> MKFYIDDLPVLFPYPKIYPEQYNYMCDIKKTLDVGGNSILEMPSGTGKTVSLLSLTIAYQMHYPEHRKIIYCSRTMSEIEKALVELENLMDYRTKELGYQEDFRGLGLTSRKNLCLHPEVSKERKGTVVDEKCRRMTNGQAKRKLEEDPEANVELCEYHENLYNIEVEDYLPKGVFSFEKLLKYCEEKTLCPYFIVRRMISLCNIIIYSYHYLLDPKIAERVSNEVSKDSIVIFDEAHNIDNVCIESLSLDLTTDALRRATRGANALDERISEVRKVDSQKLQDEYEKLVQGLHSADILTDQEEPFVETPVLPQDLLTEAIPGNIRRAEHFVSFLKRLIEYLKTRMKVLHVISETPKSFLQHLKQLTFIERKPLRFCSERLSLLVRTLEVTEVEDFTALKDIATFATLISTYEEGFLLIIEPYEIENAAVPNPIMRFTCLDASIAIKPVFERFSSVIITSGTISPLDMYPRMLNFKTVLQKSYAMTLAKKSFLPMIITKGSDQVAISSRFEIRNDPSIVRNYGSMLVEFAKITPDGMVVFFPSYLYMESIVSMWQTMGILDEVWKHKLILVETPDAQETSLALETYRKACSNGRGAILLSVARGKVSEGIDFDHQYGRTVLMIGIPFQYTESRILKARLEFMRENYRIRENDFLSFDAMRHAAQCLGRVLRGKDDYGVMVLADRRFSRKRSQLPKWIAQGLSDADLNLSTDMAISNTKQFLRTMAQPTDPKDQEGVSVWSYEDLIKHQNSRKDQGGFIENENKEGEQDEDEDEDIEMQ;> MSHSGAAIFEKVSGIIAINEDVSPAELTWRSTDGDKVHTVVLSTIDKLQATPASSEKMMLRLIGKVDESKKRKDNEGNEVVPKPQRHMFSFNNRTVMDNIKMTLQQIISRYKDADIYEEKRRREESAQHTETPMSSSSVTAGTPTPHLDTPQLNNGAPLINTAKLDDSLSKEKLLTNLKLQQSLLKGNKVLMKVFQETVINAGLPPSEFWSTRIPLLRAFALSTSQKVGPYNVLSTIKPVASSENKVNVNLSREKILNIFENYPIVKKAYTDNVPKNFKEPEFWARFFSSKLFRKLRGEKIMQNDRGDVIIDRYLTLDQEFDRKDDDMLLHPVKKIIDLDGNIQDDPVVRGNRPDFTMQPGVDINGNSDGTVDILKGMNRLSEKMIMALKNEYSRTNLQNKSNITNDEEDEDNDERNELKIDDLNESYKTNYAIIHLKRNAHEKTTDNDAKSSADSIKNADLKVSNQQMLQQLSLVMDNLINKLDLNQVVPNNEVSNKINKRVITAIKINAKQAKHNNVNSALGSFVDNTSQANELEVKSTLPIDLLESCRMLHTTCCEFLKHFYIHFQSGEQKQASTVKKLYNHLKDCIEKLNELFQDV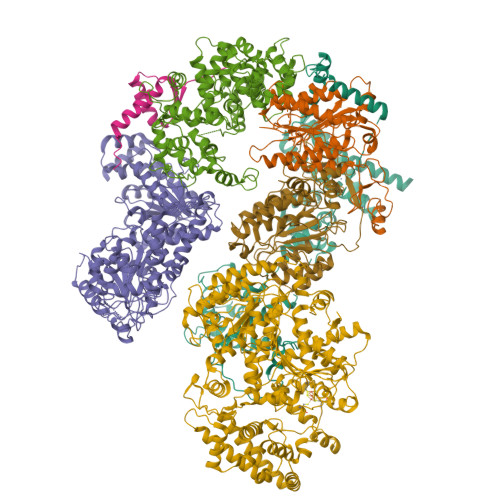LNGDGESMSNTCTAYLKPVLNSITLATHKYDEYFNEYNNNSN;> MSDYSLKHSVTQYLEEIPQQVQNRLYTSPATCLAIYRILPPLAKFFIMAMVFNENEVPLLDLDKWVNSNGKLQFQNAIKSMKSLHLLIPNKSSGTLMINLNPTFKISLRNALTGGEVQNSFGVVVEENVVSLDLLDEYSANKWETILHFMVGTPLAKIPSEKVLNLLKHSKLMEEVNSTGEFKITNEGFQFLLQEINSQLWTLLLQYLKMIETSKMDLVDVLHFIFMLGALEVGKAYKIDALSETQRIMLQDMRDYGLVFQKHSNDSIFYPTKLALMLTSDTKTIRSASNAMDSVLRQNREEPSVNEDGANGKSTTDITTSDDLNKAGLKNQDIPDGSLIVETNFKIYSYSNSPLQIAVLSLFVHLKARFVNMVLGQITRESIRRALTNGITADQIIAYLETHAHPQMRRLAEEKLEKKLELDPNCKEPLQVLPPTVVDQIRLWQLELDRVITYEGSLYSDFETSQEYNLLSKYAQDIGVLLWKDDKKKKFFISKEGNSQVLDFAKRKLKKKQ;> MDAISDPTFKHARSRKQVTEESPSLLTVIIEIAPKLWTTFDEEGNEKGSIIKVLEALIVFLNAHLAFNSANKVAVIAAYSQGIKYLYPESTSALKASESENKTRSDLKIINSDMYRRFRNVDETLVEEIYKLFELEKKQIEQNSQRSTLAGAMSAGLTYVNRISKESVTTSLKSRLLVLTCGSGSSKDEIFQYIPIMNCIFSATKMKCPIDVVKIGGSKESTFLQQTTDATNGVYLHVESTEGLIQYLATAMFIDPSLRPIIVKPNHGSVDFRTSCYLTGRVVAVGFICSVCLCVLSIIPPGNKCPACDSQFDEHVIAKLKRKPVVPRLKAKKKVTKP;> MARARKGALVQCDPSIKALILQIDAKMSDIVLEELDDTHLLVNPSKVEFVKHELNRLLSKNIYNPMDEEENQ;> MAPVVISESEEDEDRVAITRRTKRQVHFDGEGDDRVDQQQQQHSSSHRDRDKHVQRKKKKRLSNRNLQGSNGGYAWEDEIKRSWDLVKVDDEGDMASLVASIVEARKKRTAKKNITPYQRGIIRSLILTLDCSEAMLEKDLRPNRHAMIIQYAIDFVHEFFDQNPISQMGIIIMRNGLAQLVSQVSGNPQDHIDALKSIRKQEPKGNPSLQNALEMARGLLLPVPAHCTREVLIVFGSLSTTDPGDIHQTIDSLVSEKIRVKVLGLSAQVAICKELCKATNYGDESFYKILLDETHLKELFNEAVTPLPVNKINKGFTLVKMGFPTRIFEDTPTFCSCHSKLVYGGYFCPNCHSKVCSLPTVCPCCDLMLILSTHLARSYHHLMPLKTFAEVPTTEKFRSEDCFSCQSRFPILKNHKNGKLLTSSRYRCEDCKQEFCVDCDVFIHEILHNCPGCESKPVIT;> MTDVEGYQPKSKGKIFPDMGESFFSSDEDSPATDAEIDENYDDNRETSEGRGERDTGAMVTGLKKPRKKTKSSRHTAADSSMNQMDAKDKALLQDTNSDIPADFVPDSVSGMFRSHDFSYLRLRPDHASRPLWISPSDGRIILESFSPLAEQAQDFLVTIAEPISRPSHIHEYKITAYSLYAAVSVGLETDDIISVLDRLSKVPVAESIINFIKGATISYGKVKLVIKHNRYFVETTQADILQMLLNDSVIGPLRIDSDHQVQPPEDVLQQQLQQTAGKPATNVNPNDVEAVFSAVIGGDNEREEEDDDIDAVHSFEIANESVEVVKKRCQEIDYPVLEEYDFRNDHRNPDLDIDLKPSTQIRPYQEKSLSKMFGNGRARSGIIVLPCGAGKTLVGITAACTIKKSVIVLCTSSVSVMQWRQQFLQWCTLQPENCAVFTSDNKEMFQTESGLVVSTYSMVANTRNRSHDSQKVMDFLTGREWGFIILDEVHVVPAAMFRRVVSTIAAHAKLGLTATLVREDDKIGDLNFLIGPKLYEANWMELSQKGHIANVQCAEVWCPMTAEFYQEYLRETARKRMLLYIMNPTKFQACQFLIQYHERRGDKIIVFSDNVYALQEYALKMGKPFIYGSTPQQERMNILQNFQYNDQINTIFLSKVGDTSIDLPEATCLIQISSHYGSRRQEAQRLGRILRAKRRNDEGFNAFFYSLVSKDTQEMYYSTKRQAFLVDQGYAFKVITHLHGMENIPNLAYASPRERRELLQEVLLKNEEAAGIEVGDDADNSVGRGSNGHKRFKSKAVRGEGSLSGLAGGEDMAYMEYSTNKNKELKEHHPLIRKMYYKNLKK> MASTSRLDALPRVTCPNHPDAILVEDYRAGDMICPECGLVVGDRVIDVGSEWRTFSNDKATKDPSRVGDSQNPLLSDGDLSTMIGKGTGAASFDEFGNSKYQNRRTMSSSDRAMMNAFKEITTMADRINLPRNIVDRTNNLFKQVYEQKSLKGRANDAIASACLYIACRQEGVPRTFKEICAVSRISKKEIGRCFKLILKALETSVDLITTGDFMSRFCSNLCLPKQVQMAATHIARKAVELDLVPGRSPISVAAAAIYMASQASAEKRTQKEIGDIAGVADVTIRQSYRLIYPRAPDLFPTDFKFDTPVDKLPQL;> MDQNNSLPPYAQGLASPQGAMTPGIPIFSPMMPYGTGLTPQPIQNTNSLSILEEQQRQQQQQQQQQQQQQQQQQQQQQQQQQQQQQQQQQQQQQQAVAAAAVQQSTSQQATQGTSGQAPQLFHSQTLTTAPLPGTTPLYPSPMTPMTPITPATPASESSGIVPQLQNIVSTVNLGCKLDLKTIALRARNAEYNPKRFAAVIMRIREPRTTALIFSSGKMVCTGAKSEEQSRLAARKYARVVQKLGFPAKFLDFKIQNMVGSCDVKFPIRLEGLVLTHQQFSSYEPELFPGLIYRMIKPRIVLLIFVSGKVVLTGAKVRAEIYEAFENIYPILKGFRKTT;> MANSANTNTVPKLYRSVIEDVINDVRDIFLDDGVDEQVLMELKTLWENKLMQSRAVDGFHSEEQQLLLQVQQQHQPQQQQHHHHHHHQQAQPQQTVPQQAQTQQVLIPASQQATAPQVIVPDSKLIQHMNASNMSAAATAATLALPAGVTPVQQILTNSGQLLQVVRAANGAQYIFQPQQSVVLQQQVIPQMQPGGVQAPVIQQVLAPLPGGISPQTGVIIQPQQILFTGNKTQVIPTTVAAPTPAQAQITATGQQQPQAQPAQTQAPLVLQVDGTGDTSSEEDEDEEEDYDDDEEEDKEKDGAEDGQVEEEPLNSEDDVSDEEGQELFDTENVVVCQYDKIHRSKNKWKFHLKDGIMNLNGRDYIFSKAIGDAEW;> MAYQLYRNTTLGNSLQESLDELIQSQQITPQLALQVLLQFDKAINAALAQRVRNRVNFRGSLNTYRFCDNVWTFVLNDVEFREVTELIKVDKVKIVACDGKNTGSNTTE;> MGTPPGLQTDCEALLSRFQETDSVRFEDFTELWRNMKFGTIFCGRMRNLEKNMFTKEALALAWRYFLPPYTFQIRVGALYLLYGLYNTQLCQPKQKIRVALKDWDEVLKFQQDLVNAQHFDAAYIFRKLRLDRAFHFTAMPKLLSYRMKKKIHRAEVTEEFKDPSDRVMKLITSDVLEEMLNVHDHYQNMKHVISVDKSKPDKALSLIKDDFFDNIKNIVLEHQQWHKDRKNPSLKSKTNDGEEKMEGNSQETERCERAESLAKIKSKAFSVVIQASKSRRHRQVKLDSSDSDSASGQGQVKATRKKEKKERLKPAGRKMSLRNKGNVQNIHKEDKPLSLSMPVITEEEENESLSGTEFTASKKRRKH;> MAEGSRGGPTCSGVGGRQDPVSGSGGCNFPEYELPELNTRAFHVGAFGELWRGRLRGAGDLSLREPPASALPGSQAADSDREDAAVARDLDCSLEAAAELRAVCGLDKLKCLEDGEDPEVIPENTDLVTLGVRKRFLEHREETITIDRACRQETFVYE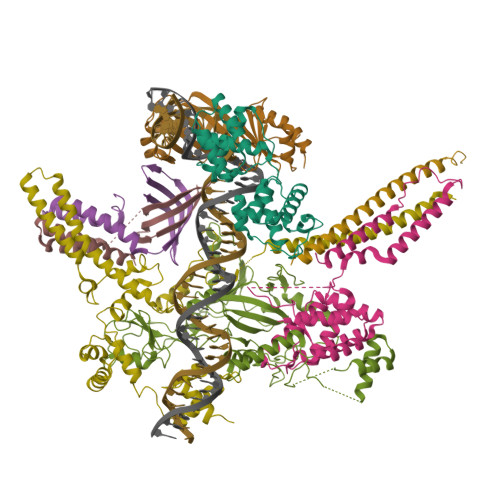MESHAIGKKPENSADMIEEGELILSVNILYPVIFHKHKEHKPYQTMLVLGSQKLTQLRDSIRCVSDLQIGGEFSNTPDQAPEHISKDLYKSAFFYFEGTFYNDKRYPECRDLSRTIIEWSESHDRGYGKFQTARMEDFTFNDLCIKLGFPYLYCHQGDCEHVIVITDIRLVHHDDCLDRTLYPLLIKKHWLWTRKCFVCKMYTARWVTNNDSFAPEDPCFFCDVCFRMLHYDSEGNKLGEFLAYPYVDPGTFN;> MDVDAEREKITQEIKELERILDPGSSGSHVEISESSLESDSEADSLPSEDLDPADPPISEEERWGEASNDEDDPKDKTLPEDPETCLQLNMVYQEVIQEKLAEANLLLAQNREQQEELMRDLAGSKGTKVKDGKSLPPSTYMGHFMKPYFKDKVTGVGPPANEDTREKAAQGIKAFEELLVTKWKNWEKALLRKSVVSDRLQRLLQPKLLKLEYLHQKQSKVSSELERQALEKQGREAEKEIQDINQLPEEALLGNRLDSHDWEKISNINFEGSRSAEEIRKFWQNSEHPSINKQEWSREEEERLQAIAAAHGHLEWQKIAEELGTSRSAFQCLQKFQQHNKALKRKEWTEEEDRMLTQLVQEMRVGSHIPYRRIVYYMEGRDSMQLIYRWTKSLDPGLKKGYWAPEEDAKLLQAVAKYGEQDWFKIREEVPGRSDAQCRDRYLRRLHFSLKKGRWNLKEEEQLIELIEKYGVGHWAKIASELPHRSGSQCLSKWKIMMGKKQGLRRRRRRARHSVRWSSTSSSGSSSGSSGGSSSSSSSSSEEDEPEQAQAGEGDRALLSPQYMVPDMDLWVPARQSTSQPWRGGAGAWLGGPAASLSPPKGSSASQGGSKEASTTAAAPGEETSPVQVPARAHGPVPRSAQASHSADTRPAGAEKQALEGGRRLLTVPVETVLRVLRANTAARSCTQKEQLRQPPLPTSSPGVSSGDSVARSHVQWLRHRATQSGQRRWRHALHRRLLNRRLLLAVTPWVGDVVVPCTQASQRPAVVQTQADGLREQLQQARLASTPVFTLFTQLFHIDTAGCLEVVRERKALPPRLPQAGARDPPVHLLQASSSAQSTPGHLFPNVPAQEASKSASHKGSRRLASSRVERTLPQASLLASTGPRPKPKTVSELLQEKRLQEARAREATRGPVVLPSQLLVSSSVILQPPLPHTPHGRPAPGPTVLNVPLSGPGAPAAAKPGTSGSWQEAGTSAKDKRLSTMQALPLAPVFSEAEGTAPAASQAPALGPGQISVSCPESGLGQSQAPAASRKQGLPEAPPFLPAAPSPTPLPVQPLSLTHIGGPHVATSVPLPVTWVLTAQGLLPVPVPAVVSLPRPAGTPGPAGLLATLLPPLTETRAAQGPRAPALSSSWQPPANMNREPEPSCRTDTPAPPTHALSQSPAEADGSVAFVPGEAQVAREIPEPRTSSHADPPEAEPPWSGRLPAFGGVIPATEPRGTPGSPSGTQEPRGPLGLEKLPLRQPGPEKGALDLEKPPLPQPGPEKGALDLGLLSQEGEAATQQWLGGQRGVRVPLLGSRLPYQPPALCSLRALSGLLLHKKALEHKATSLVVGGEAERPAGALQASLGLVRGQLQDNPAYLLLRARFLAAFTLPALLATLAPQGVRTTLSVPSRVGSESEDEDLLSELELADRDGQPGCTTATCPIQGAPDSGKCSASSCLDTSNDPDDLDVLRTRHARHTRKRRRLV;> MLSRLQELRKEEETLLRLKAALHDQLNRLKVEELALQSMISSRRGDEMLSSHTVPEQSHDMLVHVDNEASINQTTLELSTKSHVTEEEEEEEEEESDS Robo family receptors are type I transmembrane proteins that instruct neuronal wiring in various organisms, including worms, flies, mice, and humans, in addition to fulfilling diverse functions outside the nervous system. While Robo1 and Robo2 function as classical Slit receptors, the divergent family member Robo3 does not bind Slits and instead acts as a negative regulator of Robo1/2-mediated Slit repulsion. Further, a recently identified Robo3 ligand, NELL2, signals axon repulsion. NELL2 is a secreted glycoprotein containing a laminin G-like (LamG) domain, a coiled coil (CC) domain, and six epidermal growth factor-like (EGF) domains, flanked by five von Willebrand factor type C (VWC) domains.

NELL1 can bind Robo3, but it does not mediate strong commissural axon repulsion in vitro. Using SEC, we isolated a hNELL1 EGF1–3–hRobo3 FN1 complex. We crystallized and determined the structure of this complex at 1.8-Å resolution using molecular replacement (MR) with the NELL2–Robo3 model. NELL1 EGF2 also has a calcium ion bound at the conserved site observed for NELL2. The calcium ion is not directly located at the Robo3-binding site, but is still within 11 Å of the closest Robo3 atom. Second, our structural and biochemical analyses of the NELL1–Robo3 EGF1–3–FN1 complex demonstrate highly similar modes of receptor engagement by the EGF2 and EGF3 domains of the two NELL family members. First, NELL1 binds Robo3 with an affinity comparable with NELL2. Taken together, these results indicate that NELL1 and NELL2 display no significant biochemical differences in Robo3 recognition. Overall, our results indicate that NELL1 can signal through Robo3 as its receptor to induce commissural axon repulsion, albeit less effectively than NELL2. Despite these similarities, the guidance activity of NELL1 is at least one order of magnitude lower than NELL2’s.

>[3x]ADPTEPSSPPGAPSQPVVTEITKNSITLTWKPNPQTGAAVTSYVIEAFSPAAGNTWRTVADGVQLETHTVSGLQPNTIYLFLVRAVGAWGLSEPSPVSEPVRTQDSEFHHHHHH;>ADPRGHNFCAEGPKCGENSECKNWNTKATCECKSGYISVQGDSAYCEDIDECAAKMHYCHANTVCVNLPGLYRCDCVPGYIRVDDFSCTEHDECGSGQHNCDENAICTNTVQGHSCTCKPGYVGNGTICRAEFHHHHHH[3x]>XXXXXXXXXXXXXXPSNPNSPSAQLAKEEQRRKKRRLKKRIFAAVSEGCVEELVELLVELQELCRRRHDEDVPDFLMHKLTASDTGATCLMKALLNINPNTKEIVRILLAFAEENDILGRFINAEYTEEAYEGQTALNIAIERRQGDIAALLIAAGADVNAHAKGAFFNPKYQHEGFYFGETPLALAACTNQPEIVQLLMEHEQTDITSRDSRGNNILHALVTVAEDFKTQNDFVKRMYDMILLRSGNWELETTRNNDGLTPLQLAAKMGKAEILKYILSREIKEKRLRSLSRKFTDWAYGPVSSSLYDLTNVDTTTDNSVLEITVYNTNIDNRHEMLTLEPLHTLLHMKWKKFAKHMFFLSFCFYFFYNITLTLVSYYRPREEEAIPHPLALTHKMGWLQLLGRMFVLIWAMCISVKEGIAIFLLRPSDLQSILSDAWFHFVFFIQAVLVILSVFLYLFAYKEYLACLVLAMALGWANMLYYTRGFQSMGMYSVMIQKVILHDVLKFLFVYIVFLLGFGVALASLIEKCPKDNKDCSSYGSFSDAVLELFKLTIGLGDLNIQQNSKYPILFL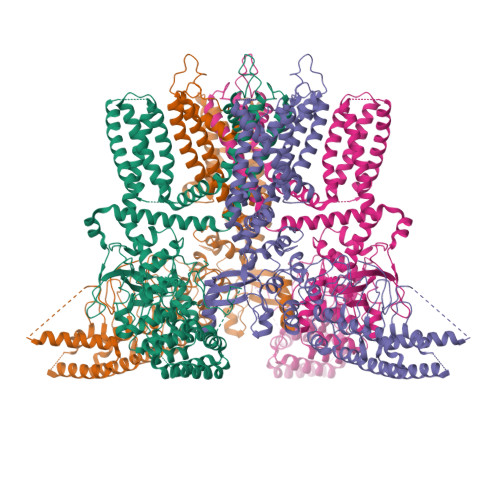FLLITYVILTFVLLLNMLIALMGETVENVSKESERIWRLQRARTILEFEKMLPEWLRSRFRMGELCKVAEDDFRLCLRINEVKWTEWKTHVSFLNEDPGPVRRTDFNKIQDSSRNNSKTTLNAFEEVEEFPETSVVDAGLEVLFQGDYKDDDDKAHHHHHH[4x]>[2x]MAKDKEFQVLFVLTILTLISGTIFYSTVEGLRPIDALYFSVVTLTTVGETPPPQTDF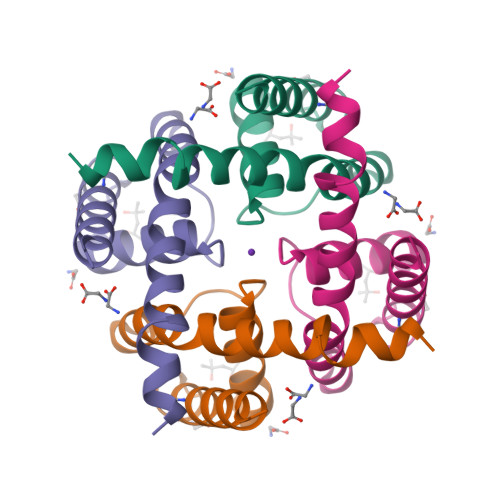GKIFTILYIFIGIGLVFGFIHKLAVNVQLPSILSNLVPR> GSTLEVRSQATQDLSEYYKGRGFE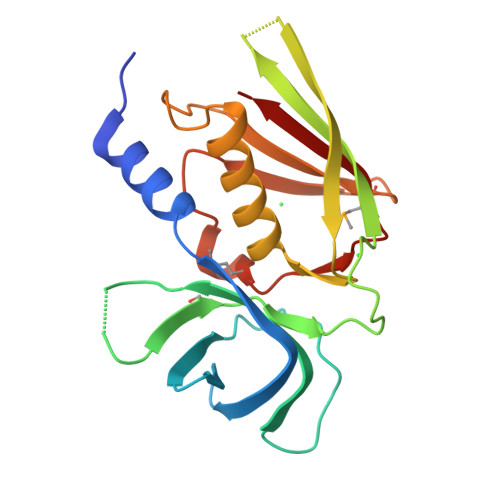LTNVTGYKYGNKVTFIDNSQQIDVTLTGNEKLTVKDDDEVSNVDVFVVREGSDKSAITTSIGGITKTNGTQHKDTVQNVNLSVSKSTGQHTTSVTSEYYSIYKEEISLKELDFKLRKHLIDKHDLYKTEPKDSKIRITMKNGGYYTFELNKKLQPHRMGDTIDSRNIEKIEVNL The stability of eukaryotic mRNAs is dependent on a ribonucleoprotein (RNP) complex of poly(A)-binding proteins (PABPC1/Pab1) organized on the poly(A) tail. This poly(A) RNP not only protects mRNAs from premature degradation but also stimulates the Pan2-Pan3 deadenylase complex to catalyze the first step of poly(A) tail shortening. Indeed, the cytoplasmic PABP interacts with and stimulates Pan2-Pan3, the deadenylase complex that trims long poly(A) tails (Uchida et al., 2004). Briefly, Pan2 wraps around an intertwined homodimer formed by two Pan3 protomers (Christie et al., 2013, Jonas et al., 2014, Schäfer et al., 2014, Wahle and Stubbs, 2014).

The cryo-EM structure of Pan2-Pan3 in complex with a poly(A) RNP composed of 90 adenosines and three Pab1 protomers shows how the oligomerization interfaces of Pab1 are recognized by conserved features of the deadenylase and thread the poly(A) RNA substrate into the nuclease active site. The resulting 3D reconstruction reached an overall nominal resolution of 4.8 Å. Pan2-Pan3 has essentially the same structure in the 90A RNP-bound state compared to the substrate-free state. The 90A RNP forms a long tubular structure that zigzags on the surface of Pan2-Pan3. Here, the conserved N-terminal edge of RRM1 packs against the conserved C-terminal α-helix of Pan2. The position of RRM1-RRM2 orients the 3′ end of the RNA at the entrance of the deadenylase cavity, which is shaped by conserved residues of the RNase and UCH-like domains. The Pab1 linker helix contacts a conserved surface of the Pan3straight pseudokinase domain, approaching the ATP-binding site. At the oligomerization interface between the first and second Pab1, the RNP density adopts a sharp V-shaped turn. At the oligomerization interface between the second and third Pab1, the RNP interacts with the WD40 domain of Pan2 at a conserved surface of the base of the β-propeller. The linker helix that extends from RRM4 of one Pab1 protomer interacts with RRM1 of the adjacent one, including a segment of the sequence preceding the RRM1 fold (referred to as leader sequence).

> MNNWQHFFNNPVDLSEHLKKPYFRFDNRDKEITAISFDEKANLIWSGDSYGCISSYDPTFQLYTRYRGHIGGNSVKDILSHRDGILSISEDSLHFANRRGVTKLNLTSIDIAAFSELNTMCYSPHSLKNNIYCGGDNTNWGIASIDLNRGCLDSLLNYSSKVKLMCSNNKVLSIGRQTGTVDLLDPTSNRTIKSFNAHSASISAMDLRDNTLVTVGKSKRFYNLYADPFVNVYDLRTMRQLPPVSFSKGTTMGSGGADFVQLHPLLPTVMIVASSSGSFDFIDLSNPTLRTQYVHPCQSIKKLCLSPNGDVLGILEADNHLDTWRRSSNNMGMFTNTPEMLAYPDYFNDITSDGPISVDDETYPLSSVGMPYYLDKLLSAWPPVVFKSEGTIPQLTGKSPLPSSGKLKSNLAVISSQNEKLSTQEFPLLRYDRTKYGMRNAIPDYVCLRDIRKQITSGLETSDIQTYTSINKYEVPPAYSRLPLTSGRFGTDNFDFTPFNNTEYSGLDPDVDNHYTNAIIQLYRFIPEMFNFVVGCLKDENFETTLLTDLGYLFDMMERSHGKICSSSNFQASLKSLTDKRQLENGEPQEHLEEYLESLCIRESIEDFNSSESIKRNMPQKFNRFLLSQLIKEEAQTVNHNITLNQCFGLETEIRTECSCDHYDTTVKLLPSLSISGINKTVIKQLNKKSNGQNILPYIEYAMKNVTQKNSICPTCGKTETITQECTVKNLPSVLSLELSLLDTEFSNIRSSKNWLTSEFYGSIIKNKAVLRSTASELKGTSHIFKYELNGYVAKITDNNNETRLVTYVKKYNPKENCFKWLMFNDYLVVEITEEEALKMTYPWKTPEIIIYCDAEELRKPFFSVDTYSINYDILFRDYFANGIRDTARREYKLLTHDEAPKSGTLVAIDAEFVSLQSELCEIDHQGIRSIIRPKRTALARISIIRGEEGELYGVPFVDDYVVNTNHIEDYLTRYSGILPGDLDPEKSTKRLVRRNVVYRKVWLLMQLGCVFVGHGLNNDFKHININVPRNQIRDTAIYFLQGKRYLSLRYLAYVLLGMNIQEGNHDSIEDAHTALILYKKYLHLKEKAIFEKVLNSVYEEGRAHNFKVPETSKG;>[3x]GPDSMADITDKTAEQLENLNIQDDQKQAATGSESQSVENSSASLYVGDLEPSVSEAHLYDIFSPIGSVSSIRVCRDAITKTSLGYAYVNFNDHEAGRKAIEQLNYTPIKGRLCRIMWSQRDPSLRKKGSGNIFIKNLHPDIDNKALYDTFSVFGDILSSKIATDENGKSKGFGFVHFEEEGAAKEAIDALNGMLLNGQEIYVAPHLSRKERDSQLEETKAHYTNLYVKNINSETTDEQFQELFAKFGPIVSASLEKDADGKLKGFGFVNYEKHEDAVKAVEALNDSELNGEKLYVGRAQKKNERMHVLKKQYEAYRLEKMAKYQGVNLFVKNLDDSVDDEKLEEEFAPYGTITSAKVMRTENGKSKGFGFVCFSTPEEATKAITEKNQQIVAGKPLYVAIAQRKDVRRSQLAQQIQARNQMRYQQATAAAAAAAAGMPGQFMPPMFYGVMPPRGVPFNGPNPQQMNPMGGMPKNGMPPQFRNGPVYGVPPQGGFPRNANDNNQFYQQKQRQALGEQLYKKVSAKTSNEEAAGKITGMILDLPPQEVFPLLESDELFEQHYKEASAAYESFKKEQEQQTEQA;> MHSLLQYHISLYAPEQPSSLKSLLKPNERSADQLFIPNNIREDLTKKNLSILQVFPSSGKVIPSIVQDYFNLVPLNFNNNDFLNKTTLFKVFSNYDGKAYVLKRLPNIDKSMNPNKISKIYQIWSKINCTNLIKFRDIFQTTKFGNLSICLVFDYYPNSLSLYDYHFVNFPKFPITNNYLWIYLVQLTNVINSIHSQNLSIGNTLNWRKVLITGDPGRIKLSHCNFMDLLFNDDTDTVVSSGGSTIEGQQQLDYKYLGELLFNLSINIENSNNNTAPKEYRLEEITPQSIDDMRQIDDKFKDVLKYLISDNGDSKKSIHDLTSHFYDKMFMVLESSQTYTEYMESVLSRELENGRLFRLVNKLNCIFGRIESRIDINWSESGTKFPIILFYDYVFHQVDSNGKPIMDLTHVLRCLNKLDAGIQEKLMLVTPDELNCIIISYKQLKDLIESTFRSITQA;> MDKINPDWAKDIPCRNITIYGYCKKEKEGCPFKHSDNTTATTINDVPPPIDVGEATTPTMTSVPKFNAKVSASFTPMTVGSDSLTTVTNTTSAATNATGNIAMAATSATASTVNPMINPIVNSSLVNNNNNNSNISISIPTTASSSNYDPFNAPIFTPSSTSSIHTNANAHSFPFPSIANSGGININATDDNSNNMSMANNVPPPMQPPPIESSNLKYPRIYPPPHSLLQYHLYAPEQPSSLKSLLKPNERSADQLFIPNNIREDLTKKNLSILQVFPSSGKVIPSIVQDYFNLVPLNFNNNDFLNKTTLFKVFSNYDGKAYVLKRLPNIDKSMNPNKISKIYQIWSKINCTNLIKFRDIFQTTKFGDLSICLVFDYYPNSLSLYDYHFVNFPKFPITNNYLWIYLVQLTNVINSIHSQNLSIGNTLNWRKVLITGDPGRIKLSHCNFMDLLFNDDTDTVVSSGGSTIEGQQQLDYKYLGELLFNLSINIENSNNNTAPKEYRLEEITPQSIDDMRQIDDKFKDVLKYLISDNGDSKKSIHDLTSHFYDKMFMVLESSQTYTEYMESVLSRELENGRLFRLVNKLNCIFGRIESRIDINWSESGTKFPIILFYDYVFHQVDSNGKPIMDLTHVLRCLNKLDAGIQEKLMLVTPDELNCIIISYKELKDLIESTFRSITQHHHHHHHHHH>[3x]MVECS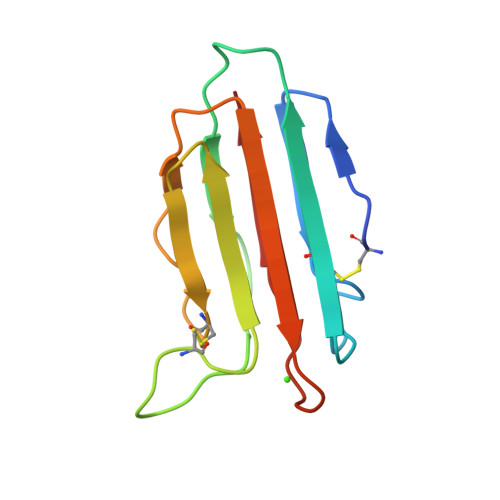GNLFTQRTGTITSPDYPNPYPKSSECSYTIDLEEGFMVTLQFEDIFDIEDHPEVPCPYDYIKIKAGSKVWGPFCGEKSPEPISTQSHSIQILFRSDNSGENRGWRLSYRA Adenosine triphosphate (ATP) synthases are multi-subunit protein complexes that use an electrochemical proton motive force across a membrane to make the cell’s supply of ATP from adenosine diphosphate (ADP) and inorganic phosphate (Pi). Proton translocation across the membrane-embedded FO region of the complex occurs via two offset half-channels. The passage of protons causes rotation of a rotor subcomplex, inducing conformational change in the catalytic F1 region to produce ATP while a peripheral stalk subcomplex holds the F1 region stationary relative to the spinning rotor during catalysis. The F1 region consists of subunits α3β3γδε, while the FO region is usually formed by three subunits with the stoichiometry ab2c9-15.

An improved map of the FO region was obtained by focused refinement of the membrane-embedded region only, excluding the soluble portion of subunit b with particle images from all three classes. In the FO region, one copy of subunit b is positioned at a location equivalent to that of the mitochondrial subunit b, while the second copy occupies the position of yeast subunit 8 (mammalian A6L) on the other side of subunit a. Multi-sequence alignment of subunit a from different species indicates that bacterial and chloroplast subunit a contain a larger periplasmic loop between α-helices 3 and 4 than found in the mitochondrial subunit. The location of the loop between α-helices 3 and 4 of the Bacillus PS3 subunit a suggests that it serves a similar structural role, compensating for the lack of subunit f in bacteria. The Bacillus PS3 ATP synthase structure implies a path for proton translocation through the bacterial complex involving two half-channels similar to the paths described for the mitochondrial and chloroplast enzymes. The cytoplasmic half-channel consists of an aqueous cavity at the interface of subunit a and the c-ring (left). The periplasmic half-channel is formed from a cavity between α-helices 1, 3, 4 and 5 of subunit a, and reaches the c-ring via a gap between α-helices 5 and 6 (right). The channels are wide and hydrophilic, suggesting that water molecules could pass freely through each of the channels before accessing the conserved Glu 56 of the c-subunits. During ATP synthesis, protons travel to the middle of the c-ring via the periplasmic half-channel and bind to the Glu 56 residue of a subunit c. Protonation of the remaining nine subunits in the c-ring returns the first glutamate to subunit a, now into the cytoplasmic half-channel, where it releases its proton to the cytoplasm due to interaction with the positively charged Arg 169 of subunit a.

> MEHKAPLVEFLGLTFNLSDMLMITITCLIVFIIAVAATRSLQLRPTGMQNFMEWVFDFVRGIINSTMDWQTGGRFLTLGVTLIMYVFVANMLGLPFSVHVNGELWWKSPTADATVTLTLAVMVVALTHYYGVKMKGASDYLRDYTRPVAWLFPLKIIEEFANTLTLGLRLFGNIYAGEILLGLLASLGTHYGVLGAVGAAIPMMVWQAFSIFVGTIQAFIFTMLTMVYMAHKVSHDH;>EAAHGISGGTIIYQLLMFIILLALLRKFAWQPLMNIMKQREEHIANEIDQAEKRRQEAEKLLEEQRELMKQSRQEAQALIENARKLAEEQKEQIVASARAEAERVKETAKKEIEREKEQAMAALREQVASLSVLIASKVIEKELTEQDQRKLIEAYIKDVQEVGGAR[2x];>[10x]MSLGVLAAAIAVGLGALGAGIGNGLIVSRTIEGIARQPELRPVLQTTMFIGVALVEALPIIGVVFSFIYLGR> CNRSCEVPTRLNSASLKQPYITQNYFPVGTVVEYECRPGYRREPSLSPKLTCLQNLKWSTAVEFCKKKSCPNPGEIRNGQIDVPGGILFGATISFSCNT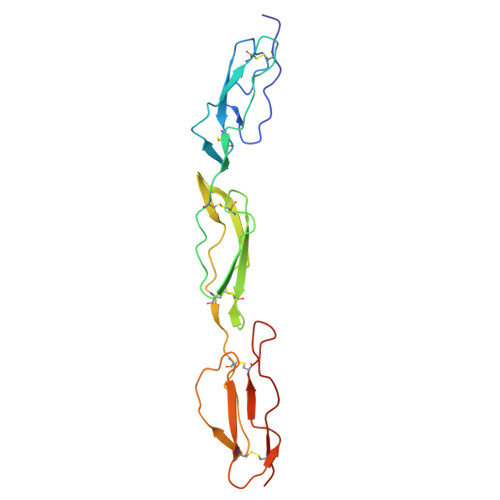GYKLFGSTSSFCLISGSSVQWSDPLPECREIYCPAPPQIDNGIIQGERDHYGYRQSVTYACNKGFTMIGEHSIYCTVNNDEGEWSGPPPECRG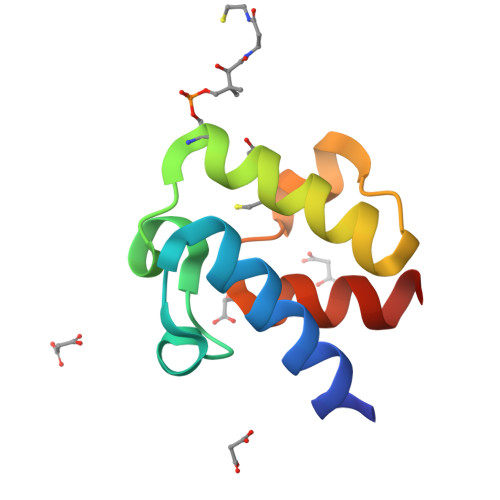>[2x]SSLKSTFDDIKKIISKQLSVEEDKIQMNSNFTKDLGADSLDLVELIMALEEKFNVTISDQDALKINTVQDAIDYIEKNNKQ>MALFGSNDVTTAHSDYEIVLEGGSSSWGKVKARAKVNAPPASPLLPADCDVKLNVKPLDPAKGFVRISAVFESIVDSTKNKLTIEADIANETKERRISVGEGMVSVGDFSHTFSFEGSVVNLFYYRSDAVRRNVPNPIYMQGRQFHDILMKVPLDNNDLIDTWEGTVKAIGSTGAFNDWIRDFWFIGPAFTALNEGGQRISRIEVNGLNTESGPKGPVGVSRWRFSHGGSGMVDSISRWAELFPSDKLNRPAQVEAGFRSDSQGIEVKVDGEFPGVSVDAGGGLRRILNHPLIPLVHHGMVGKFNNFNVDAQLKVVLPKGYKIRYAAPQYRSQNLEEYRWSGGAYARWVEHVCKGGVGQFEILYAQ[6x];>MAEQVKPAGVKPKGTVPPPKGNAPAPKANGAPGGASVIKEQDAAKMRRFLFQRTETRSTKWYQIFDTEKLDDEQVVGGHLALLGVLGFIMGIYYISGIQVFPWGAPGFHDNWFYLTIKPRMVSLGIDTYSTKTADLEAAGARLLGWAAFHFLVGSVLIFGGWRHWTHNLTNPFTGRCGNFRDFRFLGKFGDVVFNGTSAKSYKEALGPHAVYMSLLFLGWGIVMWAILGFAPIPDFQTINSETFMSFVFAVIFFALGIYWWNNPPNAAIHLNDDMKAAFSVHLTAIGYINIALGCIAFVAFQQPSFAPYYKELDKLVFYLYGEPFNRVSFNFVEQGGKVISGAKEFADFPAYAILPKSGEAFGMARVVTNLIVFNHIICGVLYVFAGVYHGGQYLLKIQLNGMYNQIKSIWITKGRDQEVQVKILGTVMALCFATMLSVYAVIVWNTICELNIFGTNITMSFYWLKPLPIFQWMFADPSINDWVMAHVITAGSLFSLIALVRIAFFAHTSPLWDDLGLKKNSYSFPCLGPVYGGTCGVSIQDQLWFAMLWGIKGLSAVCWYIDGAWIASMMYGVPAADAKAWDSIAHLHHHYTSGIFYYFWTETVTIFSSSHLSTILMIGHLVWFISFAVWFEDRGSRLEGADIQTRTIRWLGKKFLNRDVNFRFPVLTISDSKLAGTFLYFGGTFMLVFLFLANGFYQTNSPLPPPVSHAAVSGQQMLAQLVDTLMKMIA[2x];> MAEPVENKNQAPAPGAKVPPKGAPAAPKAGAPAAPKGPVAPKAGAPAAKTGASAAKQAGKPRLASLGVTLGRSGVRQE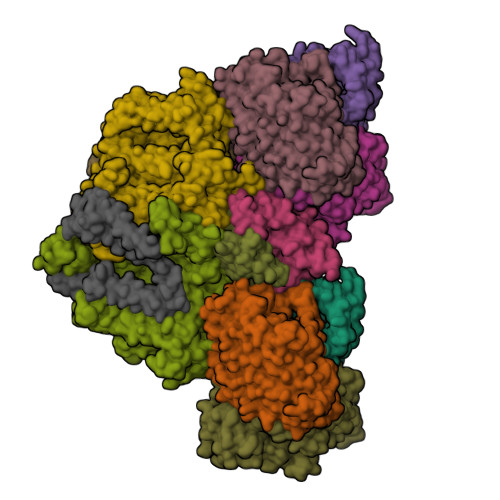SALPYVKPKAVPPPKPAAPAAKGAPAPKGAPAAPAAKAAPGAPVAKAAPKAKKHYFIIENLCVGCGLCLDKCPPKVNAIGYKFYGDVQEGGFRCYIDQAACISCSACFSGDECPSGALIEVLPDGEVLDFSYTPPERLDFDLRFLHRFHREA;>[2x]MDKNSNGKLIALAVGGAVLMGALFFSVSFLTGYIPAPNHSAILTPLRSFMGWFLLIFCASIIIMGLGKMSSAISDKWFLSFPLSIFVIVMVMFLSLRVYWEKGRTTTVDGKYIRTTAELKEFLNKPAATSDVPPAPAGFDFDAAKKLVDVRCNKCHTLDSVADLFRTKYKKTGQVNLIVKRMQGFPGSGISDDDAKTIGIWLHEKF;> MQPQLSRPQTASNQVRKAVSGPWSGNAVHKAEKYFITSAKRDRDGKLQIELVPASGRRKLSPTPEMIRRLIDGEIEIYILTTQPDIAIDMNKEIIDMENRYVIDFDKRGVKWTMREIPVFYHEGKGLCVELHNKIYTLDQFFK;> MDIRRLILAFILPPAAVMNKEAGTIMLTGILTLWGWIPGVVAALIMISKEQSGKTAEA> MSLDFNTLAQNFTQFYYNQFDTDRSQLGNL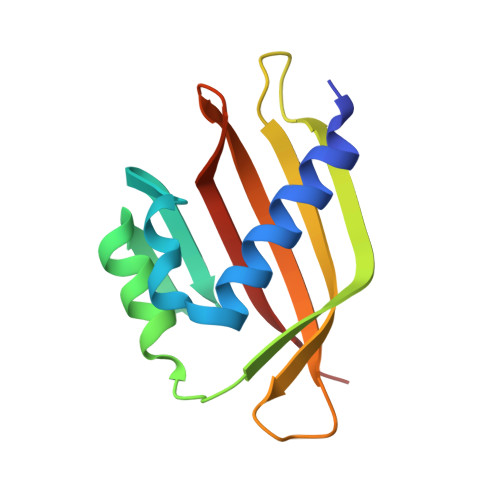YRNESMLTFETSQLQGAKDIVEKLVSLPFQKVQHRITTLDAQPASPYGDVLVMITGDLLIDEEQNPQRFSQVFHLIPDGNSYYVFNDIFRLNYSA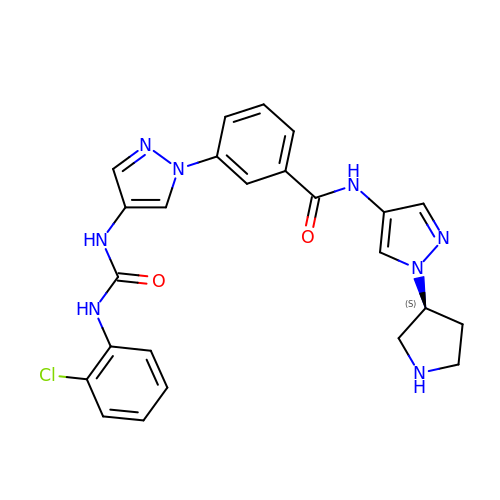3-(4-{[(2-chlorophenyl)carbamoyl]amino}-1H-pyrazol-1-yl)-N-{1-[(3S)-pyrrolidin-3-yl]-1H-pyrazol-4-yl}benzamide | C24 H23 Cl N8 O2 | IMARJVJNXLXPIX-FQEVSTJZSA-N> MAEQPPETHRFVDDYLPALLAQASQLISSEFHEVARQHGFSVSEWRVMASLAGSEPISIGQLAQVTVTKQPTVTRLLDRMEARGQVERLPHESDRRITLVRITRKGLKAVEHLMELAREHERRVLEPFGLRRAEELKQTLRQMIDLHVHVPV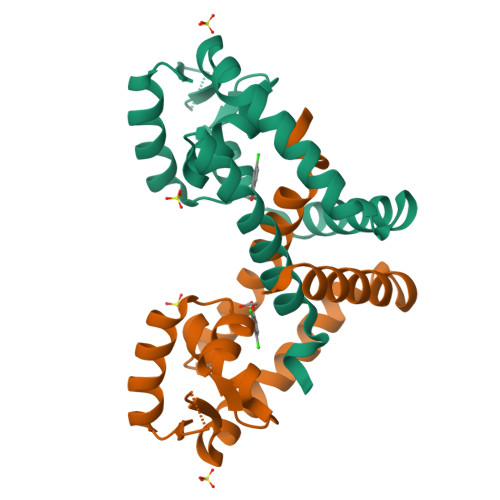EEPEED> MSASIRDAGVADLPGILAIYNDAVGNTTAIWNETPVDLANRQAWFDARARQGYPILVASDAAGEVLGYASYGDWRPFEGFRGTVEHSVYVRDDQRGKGLGVQLLQALIERARAQGLHVMVAAIESGNAASI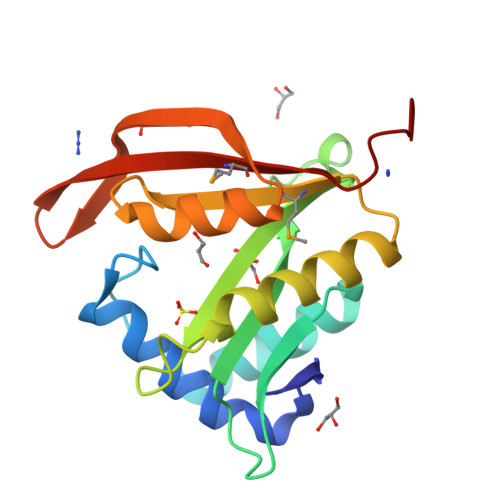GLHRRLGFEISGQMPQVGQKFGRWLDLTFMQLNLDPTRSAP(3R)-5-fluoro-3-hydroxy-1,3-dihydro-2H-indol-2-one 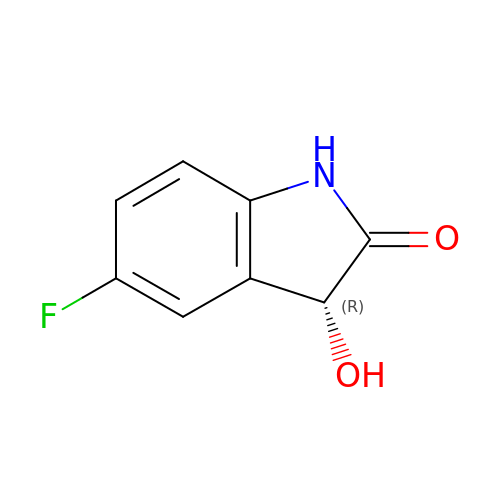| C8 H6 F N O2 | XYDTZHMQTYEJQN-SSDOTTSWSA-N>[2x]GSSPSLEQDDGDEETSVVIVGKISFCPKDVLGHGAEGTIVYRGMFDNRDVAVKRILPECFSFADREVQLLRESDEHPNVIRYFCTEKDRQFQYIAIELCAATLQEYVEQKDFAHLGLEPITLLQQTTSGLAHLHS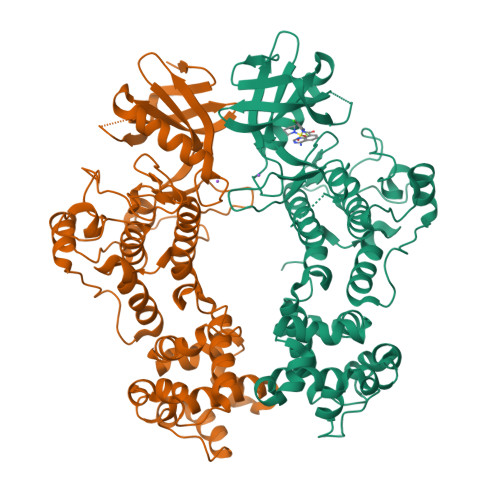LNIVHRDLKPHNILISMPNAHGKIKAMISDFGLCKKLAVGRHSFSRRSGVPGTEGWIAPEMLSEDCKENPTYTVDIFSAGCVFYYVISEGSHPFGKSLQRQANILLGACSLDCLHPEKHEDVIARELIEKMIAMDPQKRPSAKHVLKHPFFWSLEKQLQFFQDVSDRIEKESLDGPIVKQLERGGRAVVKMDWRENITVPLQTDLRKFRTYKGGSVRDLLRAMRNKKHHYRELPAEVRETLGSLPDDFVCYFTSRFPHLLAHTYRAMELCSHERLFQPYYFHEPPEPQPPVTPDAL>GSLACPEKCRCEGTTVDCSNQKLNKIPEHIPQYTAELRLNNNEFTVLEATGIFKKLPQLRKINFSNNKITDIEEGAFEGASGVNEILLTSNRLENVQHKMFKGLESLKTLMLRSNRITCVGNDSFIGLSSVRLL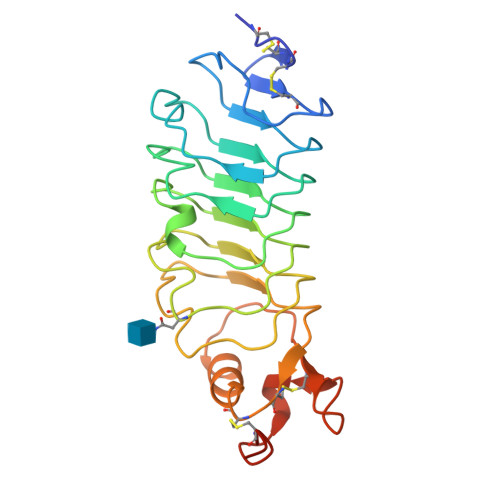SLYDNQITTVAPGAFDTLHSLSTLNLLANPFNCNCYLAWLGEWLRKKRIVTGNPRCQKPYFLKEIPIQDVAIQDFTCDDAHHHHHH[4x]>MRYRLAWLLHPALPSTFRSVLGARLPPPERLCGFQKKTYSKMNNPAIKRIGNHITKSPEDKREYRGLELANGIKVLLISDPTTDKSSAALDVHIGSLSDPPNIAGLSHFLQHMLFLGTKKYPKENEYSQFLSEHAGSSNAFTSGEHTNYYFDVSHEHLEGALDRFAQFFLSPLFDESAKDREVNAVDSEHEKNVMNDAWRLFQLEKATGNPKHPFSKFGTGNKYTLETRPNQEGIDVRQELLKFHSAYYSSNLMAVVVLGRESLDDLTNLVVKLFSEVENKNVPLPEFPEHPFQEEHLKQLYKIVPIKDIRNLYVTFPIPDLQKYYKSNPGHYLGHLIGHEGPGSLLSELKSKGWVNTLVGGQKEGARGFMFFIINVDLTEEGLLHVEDIILHMFQYIQKLRAEGPQEWVFQELKDLNAVAFRFKDKERPRGYTSKIAGILHYYPLEEVLTAEYLLEEFRPDLIEMVLDKLRPENVRVAIVSKSFEGKTDRTEEWYGTQYKQEAIPDEVIKKWQNADLNGKFKLPTKNEFIPTNFEILPLEKEATPYPALIKDTAMSKLWFKQDDKFFLPKANLNFEFFSPFAYVDPLHSNMAYLYLELLKDSLNEYAYAAELAGLSYDLQNTIYGMYLSVKGYNDKQPILLKKIIEKMATFEIDEKRFEIIKEAYMRSLNNFRAEQPHQHAMYYLRLLMTEVAWTKDELKEALDDVTLPRLKAFIPQLLSRLHIEALLHGNITKQAALGIMQMVEDTLIEHAHTKPLLPSQLVRYREVQLPDRGWFVYQQRNEVHNNSGIEIYYQTDMQSTSENMFLELFAQIISEPAFNTLRTKEQLGYIVFSGPRRANGIQGLRFIIQSEKPPHYLESRVEAFLITMEKSIEDMTEEAFQKHIQALAIRRLDKPKKLSAESAKYWGEIISQQYNFDRDNTEVAYLKTLTKEDIIKFYKEMLAVDAPRRHKVSVHVLAREMDSNPVVGEFPAQNDINLSQAPALPQPEVIQNMTEFKRGLPLFPLVKPHINFMAAKL[2x];>AAA[2x]

The proteolytic degradation and inactivation of insulin is believed to be mediated primarily by insulin-degrading enzyme (IDE), a ubiquitously expressed, soluble, secreted zinc-metalloprotease. IDE belongs to a small superfamily of zinc-metalloproteases (clan ME, family M16) that evolved independently of conventional zinc-metalloproteases. Like insulin, IDE is structurally distinctive, consisting of two bowl-shaped halves connected by a flexible linker that can switch between “open” and “closed” states. In its closed state, IDE completely encapsulates its substrates within an unusually large internal cavity that appears remarkably well-adapted to accommodate insulin.

To elucidate the mechanistic basis for these intriguing properties, we solved the co-crystal structure of Ii1 complexed to catalytically inactive, cysteine-free human IDE at 2.6-Å resolution. First, the IDE-inhibitor interaction is restricted to the catalytic zinc and subsites S1' and S2'. The P3' and P4' residues of Ii1 face the center of the catalytic chamber of IDE and do not contact IDE directly; consequently, only the main chain of these two residues could be modeled. Second, the active site of IDE is configured such that the P1' and P2' residues of Ii1 both point away from IDE's internal chamber, thereby inducing a partial turn within the amide backbone of Ii1. This partial turn, which is also present within several full-length IDE substrates, appears to be a structural prerequisite permitting extended peptides to fit within IDE's internal chamber. Finally, and quite significantly, Ii1's hydroxamate moiety, amide backbone, and P2' residue all make substantial interactions not only with residues in the N-terminal portions of IDE involved in zinc-binding and catalysis, but also with multiple residues within distal C-terminal portions of the protease. This finding highlights the fact that IDE's active site is not completely formed unless and until the N- and C-terminal portions of the protease are juxtaposed, which occurs only in the closed conformation and only during a portion of IDE's catalytic cycle. Consequently, Ii1 appears to inhibit IDE not only by active-site blockade but also by the novel mechanism of locking IDE in the closed, inactive conformation. As our co-crystal structure reveals, the potency of Ii1 can be traced to its unique ability to interact simultaneously with both the N- and C-terminal portions of the active site. Finally, and rather unexpectedly for this type of inhibitor, Ii1 proved to be remarkably selective for IDE vis-à-vis a wide range of conventional zinc-metalloproteases and representative members of other protease classes.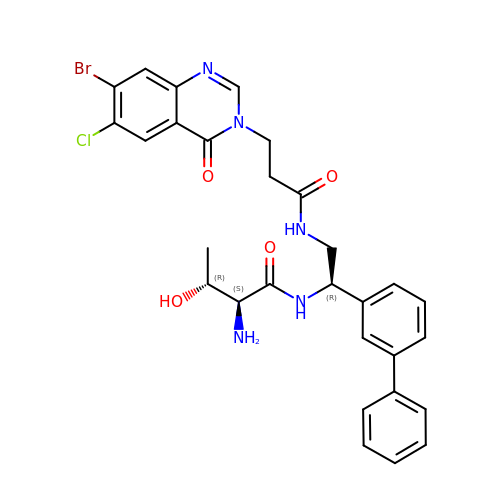(2S,3R)-2-azanyl-N-[(1R)-2-[3-(7-bromanyl-6-chloranyl-4-oxidanylidene-quinazolin-3-yl)propanoylamino]-1-(3-phenylphenyl)ethyl]-3-oxidanyl-butanamide | C29 H29 Br Cl N5 O4 | KDWXWAGYKOCBHR-ISCRSJHHSA-N>MKDRKILNEILSNTINELNLNDKKANIKIKIKPLKWKIASISLTNKTIYINKNILPYLSDEEIRFILAHELLHLKYGKYHINEFEEELLFLFPNKEAILINLINKLHQK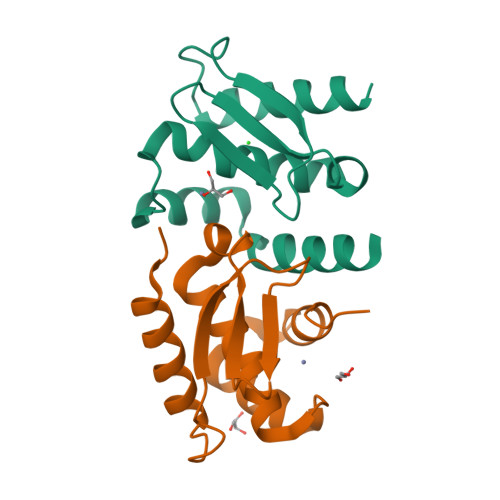K[4x]>MEELPRFFTQNGRHALLVDGAPYTILAAQLHNSSAWPAVLPPALDQVVALHANTVEAPVYWEQFEPAPGRFDTTNVDALIAGARKRGLRVALLWFGSWKNGQMHYVPEWIKRDEATYPRMRDANGEPVDVLSPHVAANVQADARAFTALMQHLRKIDGDRHTVIVVQVENEPGAIGTVRDHGPAGEAAFAQPVPAAIAAALGKPAGSWQQLFGAEAAEAFNAHATAAYIEQVAAAGKRAYPLPLYVNTWLRYKGKRYPGMDYPSGGATVNVFALWRAATPSIDFIGTDIYTSDYGEYTKVIGQYARPDNPAWVSETGFEAATAPYLFHVLGQGGIGFSVFGIDGNPDSGANRAAIAAHAAN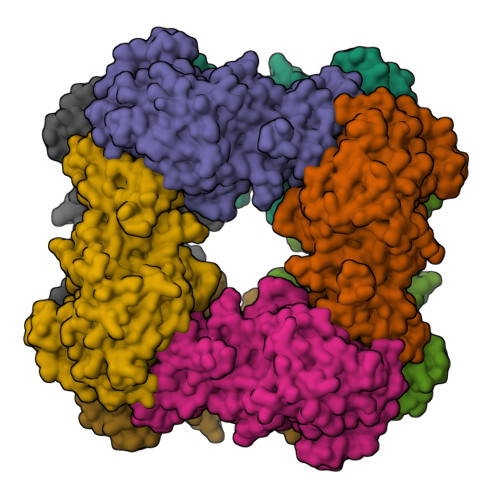FRQLAPLQRLIAQANLDGRLQAVAEQPGAPQRTLRFGDWEAKVSFGAPLWGDAPAILPGNDDHAGRLLVAQLGPEEFLVTGTAARIEFFRSAADTRHGQLLQVEQGRYVDGRWQMERQLNGDQTDYGLNFGRTDAAGQPPPVLRVRVGSY[16x]>[6x]MHRASHHELRAMFRALLDSSRCYHTASV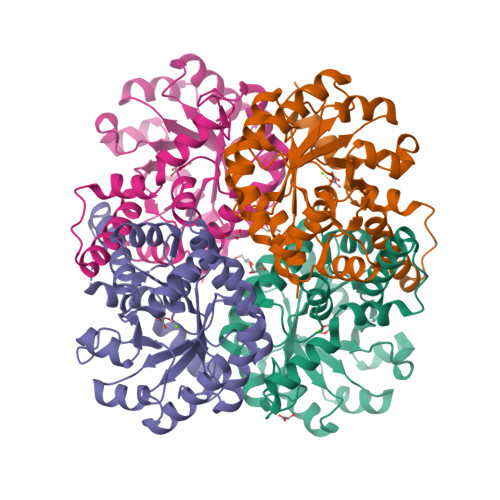FDPMSARIAADLGFECGILGGSVASLQVLAAPDFALITLSEFVEQATRIGRVARLPVIADADHGYGNALNVMRTVVELERAGIAALTIEDTLLPAQFGRKSTDLICVEEGVGKIRAALEARVDPALTIIARTNAELIDVDAVIQRTLAYQEAGADGICLVGVRDFAHLEAIAEHLHIPLMLVTYGNPQLRDDARLARLGVRVVVNGHAAYFAAIKATYDCLREERGAVASDLTASELSKKYTFPEEYQAWARDYMEVKE>[2x]XSTVHEIL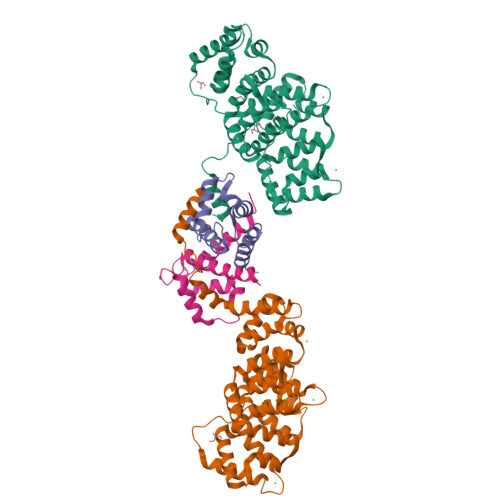CKLSLEGDHSTPPSAYGSVKAYTNFDAERDALNIETAIKTKGVDEVTIVNILTNRSNEQRQDIAFAYQRRTKKELASALKSALSGHLETVILGLLKTPAQYDASELKASMKGLGTDEDSLIEIICSRTNQELQEINRVYKEMYKTDLEKDIISDTSGDFRKLMVALAKGRRAEDGSVIDYELIDQDARDLYDAGVKRKGTDVPKWISIMTERSVPHLQKVFDRYKSYSPYDMLESIRKEVKGDLENAFLNLVQCIQNKPLYFADRLYDSMKGKGTRDKVLIRIMVSRSEVDMLKIRSEFKRKYGKSLYYYIQQDTKGDYQKALLYLCGGDD;>GSHMACPLEKALDVMVSTFHKYSGKEGDKFKLNKSELKELLTRELPSFLGKRTDEAAFQKLMSNLDSNRDNEVDFQEYCVFLSCIAMMCNEFFEGFPDKQPRKK[2x]>MRVLGIDPGLANLGLGLVEGDVRRAKHLYHVCLTTESAWLMPRRLQYLHEELTRLLTEYRPDAVAIEDQILRRQADVAFKVGQAFGVVQLACAQAGVPIHAYGPMQVKKSLVGTGRADKEQVIYMVKASLGIRELFNNHAADALALALTHLAHAPMQERSERLAAAGRAAR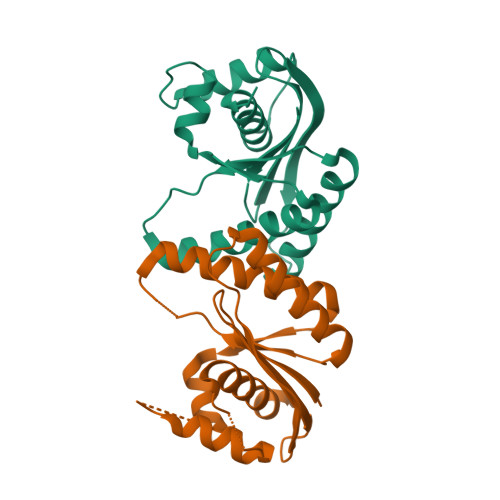TGDAPLRR[2x]>[4x]MTTPISPPPQWSRRRQEKQRRLE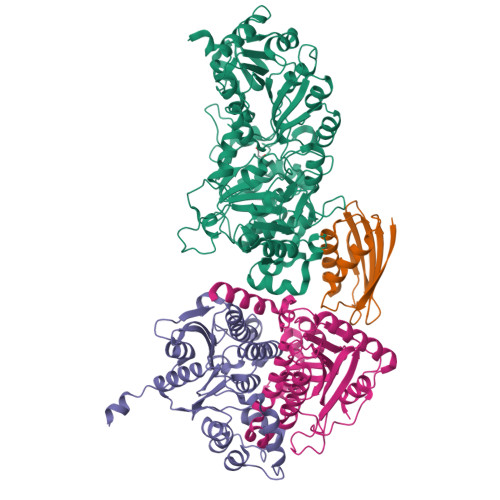RVRGLADGAVLPREGLVAALEALIAPGDRVVLEGNNQKQADFLSRSLARVDPGKLHDLHMIMPSVGRPEHLDLFELGIARKLDFSFSGPQSLRIGQLLEDGLLEIGAIHTYIELYARLVVDLIPNVALVAGFVADREGNVYTGPSTEDTPALVEPTAFSDGIVIVQVNRIVDDPRDLPRVDIPASWVDFVVEADQPFYIEPLFTRDPRHIKPVHVLMAMMAIRGIYQRHNVQSLNHGIGFNTAAIELILPTYGESLGLKGKICRHWTLNPHPTLIPAIESGWVESVHCFGTELGMEGYIAQRPDVFFTGRDGSLRSNRMFCQLAGQYAVDLFIGATLQVDGDGHSSTVTRGRLAGFGGAPNMGHDPRGRRHSTPAWLDMRGEPEALLERGRKLVVQMVETFQDGGKPTFVERLDALEVARQTGMPLAPVMIYGDDVTHVLTEEGIAYLYKARSLEERQAMIAAVAGISPIGLRHDPRETQRMRREGLIALPEDLGIRRTDASRELLAAKSIAELVEWSGGLYQPPARFRSW;>METLSFEFPAGQPGRGRALVGCVGSGDLEVLLEPGQPGKLSIQVQTSVNGSASRWQHLFERLFDGQTPPALLIDIHDFGATPGVVRLRLEQGFEEIGHD[4x];>MTDVARLLALRSFTELGARQRARALLDAGSFRELLDPFAGVQSPWLERQGIVPQADDGVVVARGLLDGQPAVLAAIEGAFQGGSLGEVSGAKIAGALELAAEDNRNGVPTRALLLLETGGVRLQEANLGLAAIAEIQAAIVDLQRYQPVVAVIAGPVGCFGGMSIAAGLCSYVLVTREARLGLNGPQVIEQEAGIAEYDSRDRPFIWSLTGGEQRFASGLADAYLADDLDEVRTSVLAYFAKGLPARPRCRRAEDYLRRLGDLDTAEQPDAAGVRRLYQGLGQGDAT[4x];>MGSSHHHHHHSQDPNSMSQPFASRGLAWFQALAGSLAPRPGDPASLRVADAELDGYPVRFLAVVPDPDNPFPRARQGEVGLLEGWGLAAAVDEALEADREAPRKRALLAIVDVPSQAYGRREEALGIHQALAGAVDAYARARLAGHPLIGLLVGKAMSGAFLAHGYQANRLIALHDPGVMVHAMGKAAAARITLRSVEELEALAAKVPPMAYDIDSYASLGLLWRTLPVETVEVPSTADLVRVRTCLGEALADILGGPRDLGGRLGAANREASARVRRLLREQW[4x]> GQVIVV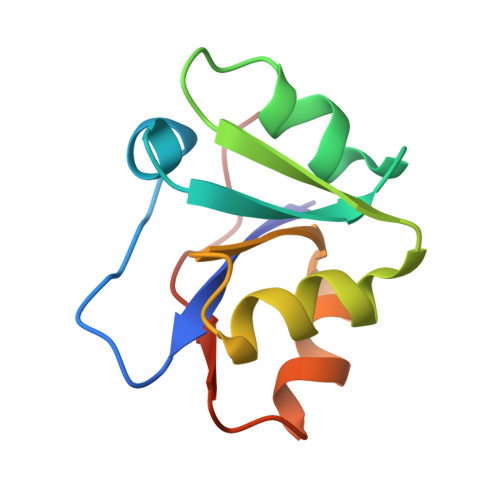RKDSDFRPKTYEDLVGKTVAVQIGTTGDIEVSKYDGIKVVRFDKFTDAFLELKRGRADAVVLDSATARAFVAKNPDLVISSGVLSS> NGIVPDAGHQGPDVSAVNGGTQVINIVTPNNEGISHNQYQDFNV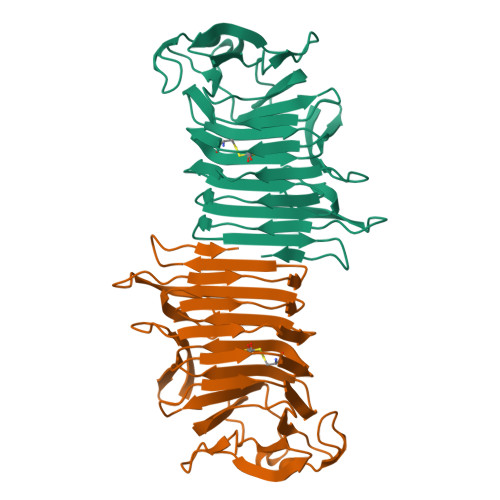GKPGAVFNNALEAGQSQLAGHLNANSNLNGQAASLILNEVVSRNPSFLLGQQEVFGIAAEAVLSNPNGITCDGCGFINTSRSSLVVGNPLFENGQLKGYSTLNNTNLLSLGKNGLNTTGLLDLIAPRIDSRGKITAAEISAFTGQNTFSQHFDILSSQKPVSALDSYFFGSMQSGRIRIINTAEGSGVKLAGHHHHHH>[6x]MISATRLQRAVRPAARAFSQSANPSRILVTGGTGQI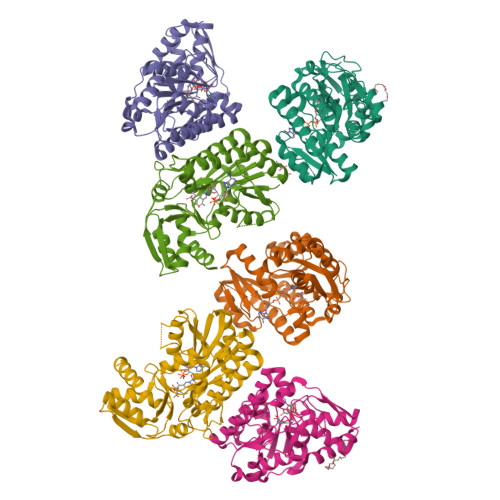GMELVPYMRQLFGADTIVNSDIKAPGGGHRDGNFVYCDVQDRDSMARIVTEQGVDTIVHMASLLSAVGEANPSLALSVNTRGIQNVLELAKQYQLRVFAPSTIAVFGPSTPQDETPDTTIMRPTTMYGLTKVHVELLGEYYYNKFGVDFRSVRYPGVISSEALPGGGTTDYAVEIFYEALKHGKYTCFLNRDAKLPMMYMPDCLKATMGLINAPNDCLSQRTYNITAVSFTPEEIVASIQKVMPSFQCDYKPDFRQQIAETWPRSIDDSIARKDWNWQHDFDLDSMVEDMLVKLDAKLSKPEAAVEETA> MSSLKLYHFPVSGPSRGALLAARAIGIPIQIEIVNLFKKEQLQESFLKLNPQHCVPTLDDNNFVLWESRAIACYLADKYGKDDQWYPKDLQKRAVVNQRLYFDSASLYVKIRAICFPILFLGETEIKQSLKDDLNSTLSFLNQFLEKTKWVAADHP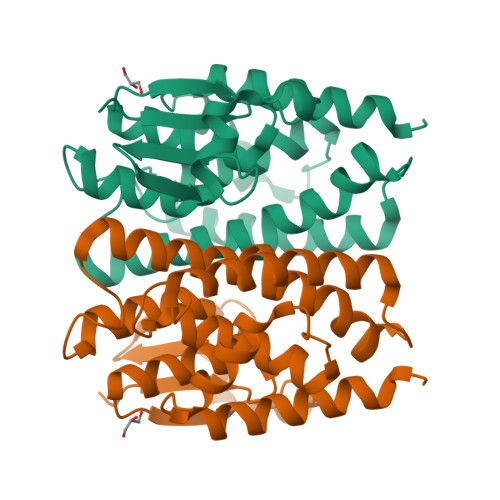TIADTSIYASMSSILAVGWDISSFPNIQRWIKDCLLLPGAPENEDGARTFGDAVKKNIKQ(3S)-3-hydroxybutyl beta-D-xylopyranoside 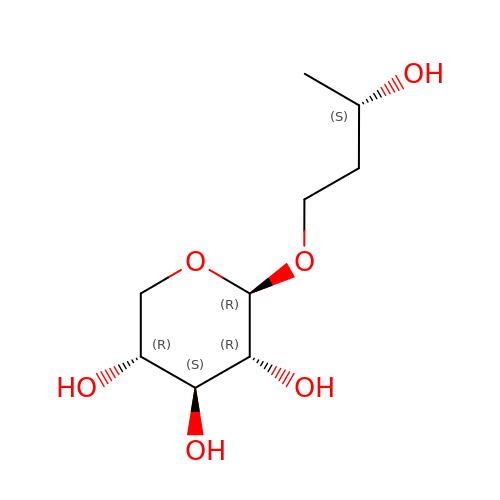| C9 H18 O6 | KAKVKOIRYXYSBS-KVEIKIFDSA-N> MLFRSVSCKNYQRGGWSPGSKHQKHMTLNPTLYLYRFPGPHGPGPYTMKYWWTLGCFPTGMEVPFRLHEFLSTYQQEHVPVEVEEWLRCYIKDPLSELVNASNDFFKAVEVYPEVESARGYKTLQPSIAPLLVPMKKFEEQLGVKISPVGLRSVLSNPVLKDRFLDDLFDYKSYVEKGGSTPHRRLARSRFEGSLSVLGECEKCLPEQHQVEISESLGTFIGATVSPAETTADDERSLILLLTTISEGCINAGNYSDAASVLADALMFCHDPDSQATTHANISFASLLNADFKGAEYNGREAALLQPQVKPTSTACARGYVGWAAAAAYQDDFEKAEAIVKDGLTLYVGNEHLEKLANKLQALREEQPSVYKQVPRSLRESRSHLPSQQSRGLLSGSGKGFS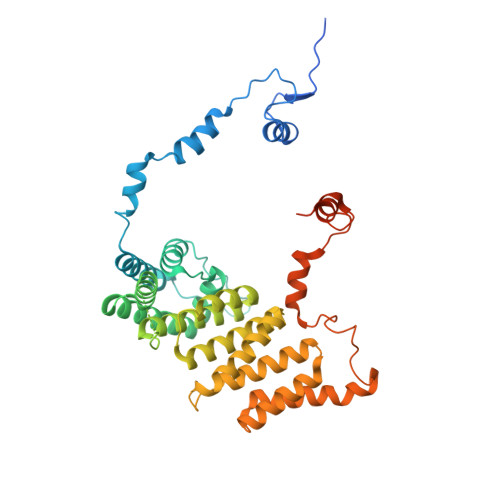NEFDWVEFKNKLYPSKMDPRNNEMGSVFRRVGDLGSFISTSRSMERL(((R)-1-(((benzyloxy)carbonyl)amino)-2-phenylethyl)oxidophosphoryl)glycyl-L-leucinate 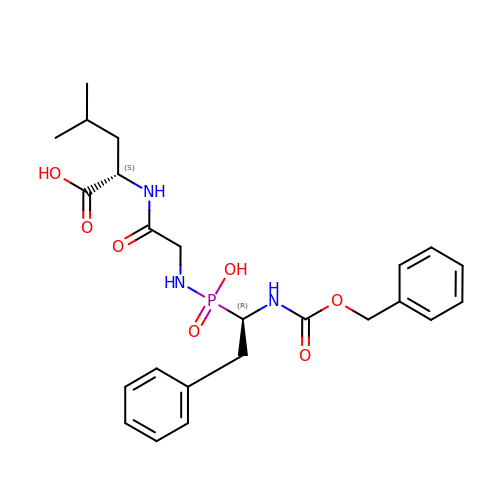| C24 H32 N3 O7 P | YJSHTZYDPJRJOL-RBBKRZOGSA-N> MQKEQLSALMDGETLDSELLNELAHNPEMQKTWESYHLIRDSMRGDTPEVLHFDISSRVMAAIEEEPVRQPAT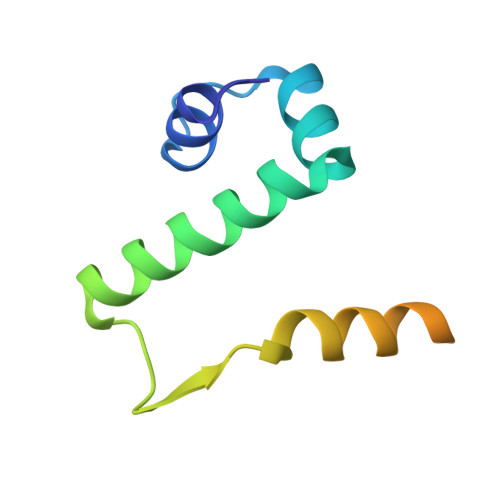LIPEAQPAPHQWQKMPF4-azanyl-2-sulfanyl-benzoic acid | C7 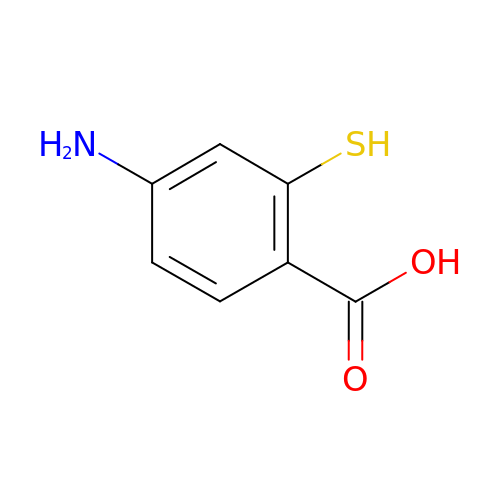H7 N O2 S | QTXSDPJOPCWEME-UHFFFAOYSA-N>[4x]MASMTGGQQMGRGSMKKLVVITGASSGIGEAIARRFSEEGHPLLLLARRVERLKALNLPNTLCAQVDVTDKYTFDTAITRAEKIYGPADAIVNNAGMMLLGQIDTQEANEWQRMFDVNVLGLLNGMQAVLAPMKAR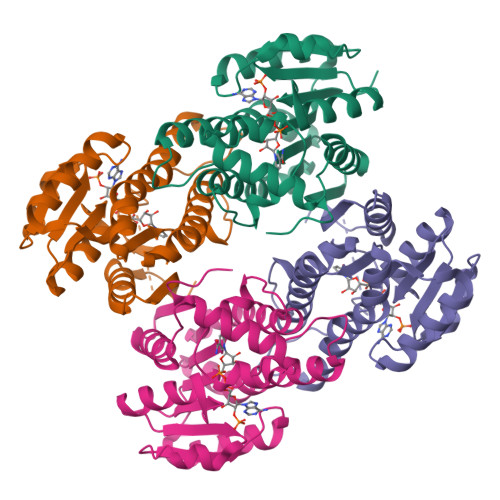NCGTIINISSIAGKKTFPDHAAYCGTKFAVHAISENVREEVAASNVRVMTIAPSAVKTELLSHTTSQQIKDGYDAWRVDMGGVLAADDVARAVLFAYQQPQNVCIREIALAPTKQQPKLAAALEHHHHHH>MLIAFEGIDGSGKTTQAKKLYEYLKQKGYFVSLYREPGGTKVGEVLREILLTEELDERTELLLFEASRSKLIEEKIIPDLKRDKVVILDRFVLSTIAYQGYGKGLDVEFIKNLNEFATRGVKPDITLLLDIPVDIALRRLKEKNRFENKEFLEKVRKGFLELAKEEEN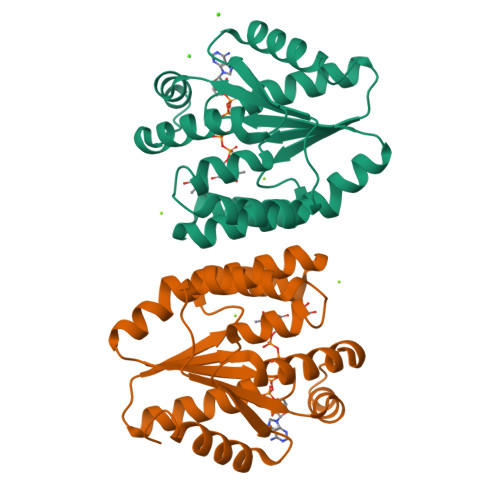VVVIDASGEEEEVFKEILRALSGVLRV[2x]Import of proteins into peroxisomes depends on PEX5, PEX13 and PEX14. By combining biochemical methods and structural biology, we show that the C-terminal SH3 domain of PEX13 mediates intramolecular interactions with a proximal FxxxF motif. The SH3 domain also binds WxxxF peptide motifs in the import receptor PEX5, demonstrating evolutionary conservation of such interactions from yeast to human. Strikingly, intramolecular interaction of the PEX13 FxxxF motif regulates binding of PEX5 WxxxF/Y motifs to the PEX13 SH3 domain.

In this study, we present a high-resolution structure of the human PEX13 SH3 domain with an intramolecular FxxxF motif, demonstrating the structural basis of this non-canonical interaction with an SH3 domain. The domain boundaries defined by the NMR analysis were used to generate chimeric constructs which contain the PEX13 SH3 domain and the FxxxF motif (D371EQEAAFESVFV383) separated by GGGGS (GS) linkers. Structures of the apo SH3 domain and SH3-(GS)2-FxxxF were solved by X-ray crystallography at 1.8Å and 2.3Å resolution, respectively. The structure of the complex shows interactions of the α-helical FxxxF motif and SH3 domain mediated by hydrophobic contacts of the two phenylalanines, which clamp around β1 and β5, and polar interactions involving sidechain and backbone contacts. Backbone hydrogen-bonds are formed between A376 and G335 as well as S379, F381 and K336. The negatively charged sidechains E374 and E378 show electrostatic interactions with K304, E305, K336, and a water molecule. Interestingly, nine out of the eleven Arg and Lys residues are located at the FxxxF binding surface, forming a positively charged surface area, which is favorable for binding negatively charged peptides such as the C-terminal FxxxF motif. The crystal structure was confirmed in solution by NMR titration experiments of the isolated SH3 domain with an FxxxF peptide (350-403). Strong chemical shift perturbations map to the binding site seen in the crystal structure, and spectral changes at saturated binding are very similar to the native SH3-CTR protein.

>VTDSINWASGEDDHVVARAEYDFAAVSEEEISFRAGDMLNLALKEQQPKVRGWLLASLDGQTTGLIPANYVKILGKRKGRKTVESSGGGGSGGGGSDEQEAAFESVFVE[2x]> SNAAPKSLDATPVDAQLLKFGMSTALSGPAAELGINMRHGILAAFDEAKAKNHLPSKTLKLIALDDGYEPARTAPNMHRLTDEHEVLAVVGNVGTPTAITAIPIAQQTKTPFFGAFTGASALRKTESVEFVINYRASYAEETAAMVDALVAKGIKPEEIGFFTQNDSYGDDGFFGGLAAIRRHQSVKVSSLPHGRYRRNTSQVEDGLADLLMHQPLPKAVIMVGTYEPCSKLIRMARMNNFNPQFLAVSFVGADALQRSLGDLANGIVATQVVPH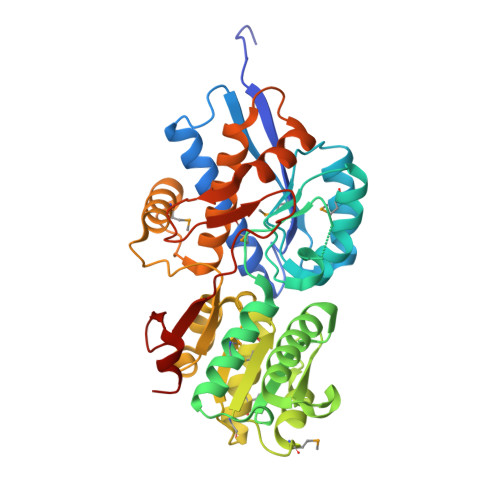FDSDLPLVREYRDAMRDYDPELPLSFVSLEGYIVGRILVKAVTSIKGEISRSSIAAALEQLGQFDIGLGAPLTLGPNDHQASSKVWPVLIGADSSQSLAWEELLSE>MSLPMLQVALDNQTMDSAYETTRLIAEEVDIIEVGTILCVGEGVRAVRDLKALYPHKIVLADAKIADAGKILSRMCFEANADWVTVICCADINTAKGALDVAKEFNGDVQIDLTGYWTWEQAQQWRDAGIGQVVYHRSVDAQAAGVAWGEADITAIKRLSDMGFKVTVAGGLALEDLPLFKGIPIH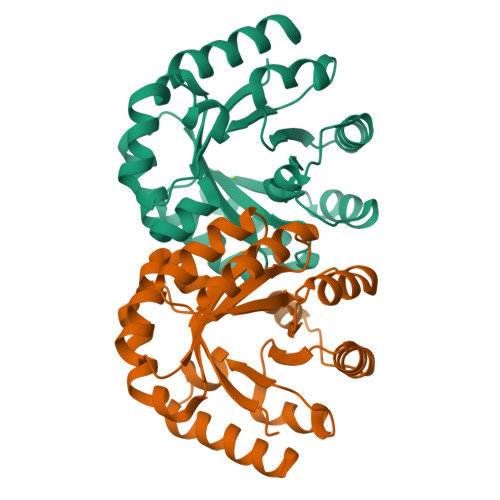VFIAGRSIRDAASPVEAARQFKRSIAELWG[2x]> SKTAKIDWSHWTVTVPEENPDKPGKPYSLGYPEILNYAEDKIASKYMYDDPKDKSVVFYAFPSGVTTANTHYSRSELRETMETGSNKVNWTFAKGGKMRGTYAIDDISKEPDG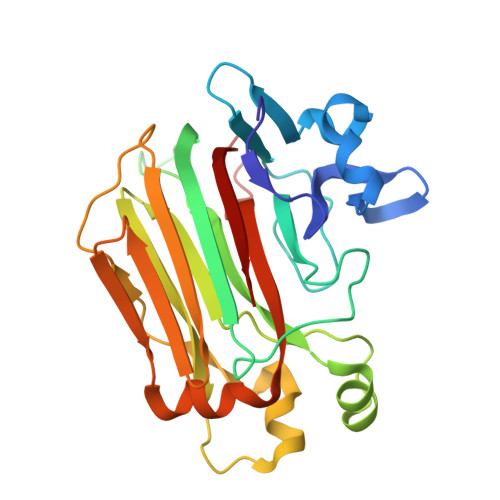KYSRVIIAQIHGVLTDEQRDLIGQKDNNAPPILKVYWDKGKIRVKTKVLKDLNAPYKEMLSEHAWGDDEGRNFKEKIDLNTRFTLEVKVSDGRMEVILNDTESLVYDDIHMKKWGIFENYFKAGNYFQSKTPGTFAKVKIYSLQVTH>NTGELKNLNEKYEQLSQYLNQVASLKQSIQNANNIELVNSSLNYLKSFTNNNYNSTTQSPIFNAVQAVITSVLGFWSLYAGNYLTFFVVNKDTQKPASVQGNPPFSTIVQNCSGIENCAMNQTTYDKMKKLAEDLQAAQQNATTKANNLCALSGCATTQGQNPSSTVSNALNLAQQLMDLIANTKTAMMWKNIVIAGVSNVSGAIDSTDYPTQYAVLNNIKAMIPILQQAVTLSQSNHTLSASLQAQATGSQTNPKFAKDI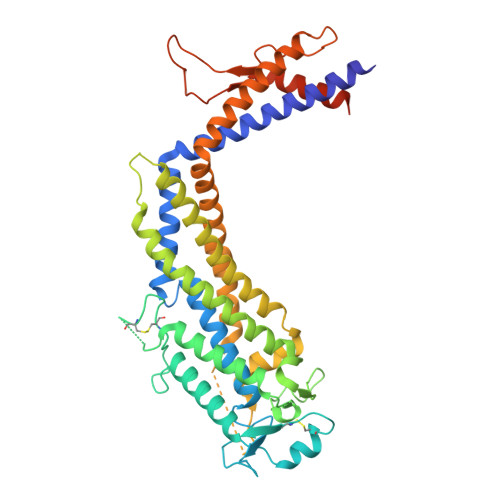YAFAQNQKQVISYAQDIFNLFSSIPKDQYRYLEKAYLKIPNAGKTPTNPYRQEVNLNQEIQTIQNNVSYYGNRVDAALSVAKDVYNLKSNQTEIVTTYNNAKNLSQEISKLPYNQVNTKDIITLPYDQNAPAAGQYNYQINPEQQSNLSQALAAMSNNPFKKVGMISSQNNNGHHHHHH[2x]>SNAMSYAKEIDTLNQHIADFNKKINVSFEFFPPKNEKMETLLWDSIHRLKVLKPKFVSVTYGANSGERDRTHGIVKAIKQETGLEAAPHLTGIDATPEELKQIARDYWDSGIRRIVALRGDEPKGY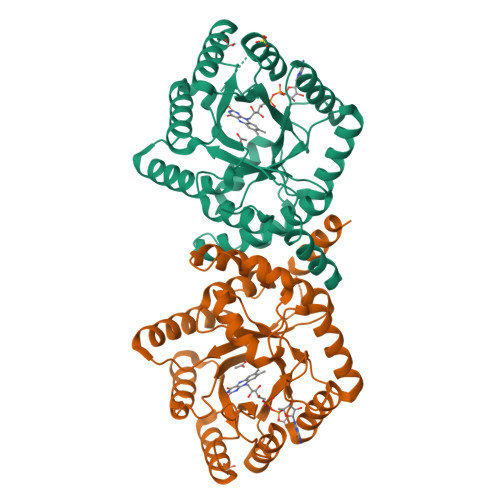AKKPFYASDLVELLRSVADFDISVAAYPEVHPEAKSAQADLINLKRKIDAGANHVITQFFFDIENYLRFRDRCASIGIDTEIVPGILPVTNFKQLQKMASFTNVKIPAWLVKAYDGLDNDPTTRNLVAASVAMDMVKILSREGVNDFHFYTLNRSELTYAICHMLGVRP[6x]> ITGTSTVGVGRGVLGDQKNINTTYSTYYYLQDNTRGNGIFTYD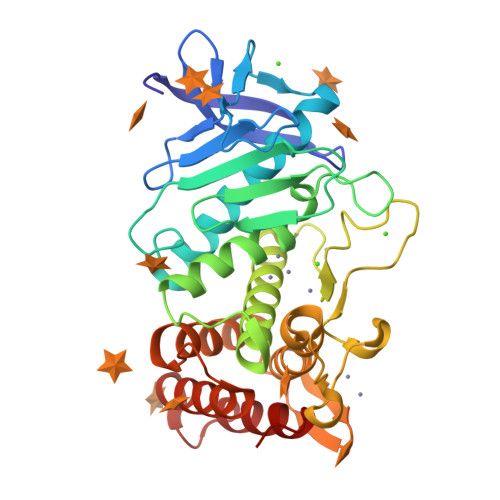AKYRTTLPGSLWADADNQFFASYDAPAVDAHYYAGVTYDYYKNVHNRLSYDGNNAAIRSSVHYSQGYNNAFWNGSQMVYGDGDGQTFIPLSGGIDVVAHELTHAVTDYTAGLIYQNESGAINEAISDIFGTLVEFYANKNPDWEIGEDVYTPGISGDSLRSMSDPAKYGDPDHYSKRYTGTQDNGGVHINSGIINKAAYLISQGGTHYGVSVVGIGRDKLGKIFYRALTQYLTPTSNFSQLRAAAVQSATDLYGSTSQEVASVKQAFDAVGVK>[2x]AEKQAKINRREEILQALAEMLESNEGASRITTAKLAKQVGVSEAALYRHFPSKTRMFEGLIEFIEESLMSRINRIFDEEK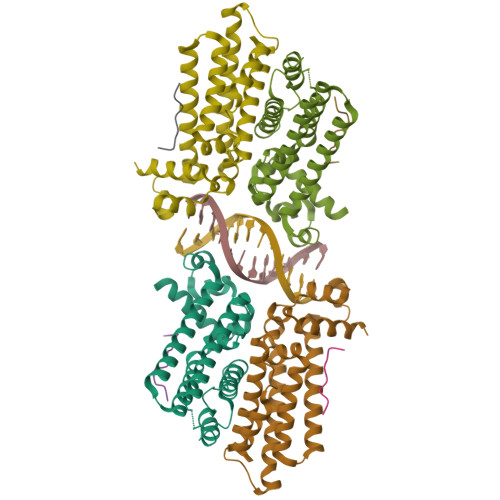DTLNRIRLVMQLLLAFAERNPGLTRILSGHALMFENERLRDRINQLFERIETSLRQILRERKLREGKSFPVDENILAAQLLGQVEGSLNRFVRSDFKYLPTANFDEYWALLSAQIK;>DYLDIPAFLR[2x]Here we report seven high-resolution cryo-EM structures of filamentous peptide nanotubes based on a cross-α supramolecular architecture that provide insight into the designability of helical peptide filaments. A structural interaction is identified based on an appropriately placed pair of arginine residues (RxxxR) within the corresponding peptide sequences. This local interaction motif, designated as an arginine clasp, is robust within the context of these cross-α assemblies and can guide the coalescence of helical protofilaments into structurally defined cross-α nanotubes. In contrast to most structurally characterized filaments based on synthetic α-helical coiled-coils, the chain axes of the helical protomers are oriented in a plane nearly perpendicular to the long axis of the assembly.

Therefore, the designed series of Form I-like peptides encompassed minimal peptide sequences in which the structurally determinative distance between the RxxxR motif and the C-terminus was systematically varied over the range from 2 to 5 heptad repeats. Three filaments, derived from peptides 15-10-3, 29-24-3, and 36-31-3, were selected for further analysis using cryo-EM imaging with direct electron detection. Five protofilaments interacted to form the 15-10-3 filament, four interacted in the 29-24-3 filament, and three interacted in the 36-31-3 filament. The Form I/29-17-3 structure fits the observed trend, in that the 17 amino acid length of the structurally determinative segment lay between the 10 amino acid and 24 amino acid segment length of 15-10-3 and 29-24-3, respectively. Similarly, the 4-start helices of 29-17-3 and 29-24-3 and the 3-start helices of 36-31-3, passing through every fourth subunit and every third subunit, respectively, were associated with the axial stacking direction of the protofilaments within the corresponding assemblies. For the 29-24-3 peptide, the interaction occurred between the C-terminus of peptide (ia) and the RxxxR motif of peptide (ib + 1), in contrast to the C5-symmetric structure of 15-10-3 that involved helices ia and ib. First, the tilt angle of the core peptide with respect to the plane normal to the filament axis became progressively more negative with increasing peptide length. Despite the differences in cross-sectional geometry for the respective filaments, the helix crossing angles were remarkably similar and lay within the range from 95° to 105°. The length and flexibility of the arginine side-chains enabled the conservation of the RxxxR lateral interaction between protofilaments despite differences in peptide length.

>[40x]QAEILRAYARILEADAKILEAHAEILKAQ The crystal structure of Dhaf4260 from Desulfitobacterium hafniense DCB-2 was determined by single-wavelength anomalous diffraction (SAD) to a resolution of 2.01 Å using the semi-automated high-throughput pipeline of the Joint Center for Structural Genomics (JCSG) as part of the NIGMS Protein Structure Initiative (PSI). This protein structure is the first representative of the PF04016 (DUF364) Pfam family and reveals a novel combination of two well known domains (an enolase N-terminal-like fold followed by a Rossmann-like domain). Structural and bioinformatic analyses reveal partial similarities to Rossmann-like methyltransferases, with residues from the enolase-like fold combining to form a unique active site that is likely to be involved in the condensation or hydrolysis of molecules implicated in the synthesis of flavins, pterins or other siderophores. The genome context of Dhaf4260 and homologs additionally supports a role in heavy-metal chelation. The Dhaf4260 protein family DUF364 (PF04016) contains around 165 homologs that are mostly found in cyanobacteria, actinobacteria, thermotogae and proteobacteria, but are also found in firmicutes and a range of archaea; all of these proteins are approximately 230 residues in length.

The final model includes two Dhaf4260 protomers [491 residues; molecule A contains residues 1–102 and 110–251 in addition to three residues from the N-terminal expression and purification tag (residues −2A to 0A), and molecule B contains residues 1–102 and 115–251 and five residues from the N-terminal expression and purification tag (residues −4B to 0B)], six ethylene glycol molecules, four imidazole molecules, two chloride ions and 239 water molecules in the asymmetric unit. The electron density was insufficient to model the loop connecting the N- and C-terminal domains (residues 103–109 in molecule A and residues 103–114 in molecule B) and the remainder of the N-terminal expression and purification tags (residues −18 to −3 in molecule A and −18 to −5 in molecule B). Dhaf4260 is a two-domain α+β protein. Size-exclusion chromatography of Dhaf4260 in combination with static light scattering indicates a mixture of oligomerization states, with a tetramer being the predominant quaternary form. However, crystal-packing analysis of the Dhaf4260 structure only supports a monomer or dimer and did not identify any higher order oligomeric state in this crystal form. The presence of the 19-residue N-terminal expression and purification tag might also alter the oligomerization state relative to the wild-type protein. In addition, the Dhaf4260 pocket is both narrower and longer than in Rossmann-like methyltransferases such as MT0146, suggesting that it catalyzes the modification of a longer substrate or the condensation of two molecules. A chloride ion is present in this cleft in both molecules in the asymmetric unit and is coordinated by the backbone amide of Trp149 and solvent.

>[2x]MGSDKIHHHHHHENLYFQGMWEIYDAMINGIPEDFLVDELVCGTTHSVIRSGNGVGLGPNRPFETRMPMLTQNLLGLPLRVAAGCVKSWNYVEASIGLAAINAYYNNPQVAREHGVIFSDAKRVEDRMNDPFIMSQNEVKGKKVGVVGHFPHLESLLEPICDLSILEWSPEEGDYPLPASEFILPECDYVYITCASVVDKTLPRLLELSRNARRITLVGPGTPLAPVLFEHGLQELSGFMVKDNARAFRIVAGAEKVKIYSAGQKVTIKK>GGHMKNILVTGGLGFIGSNFVNHISSKYDNVNIYVYDIGDYCASVENVEWNNRTKLIKGDIRNFDLIMHTLT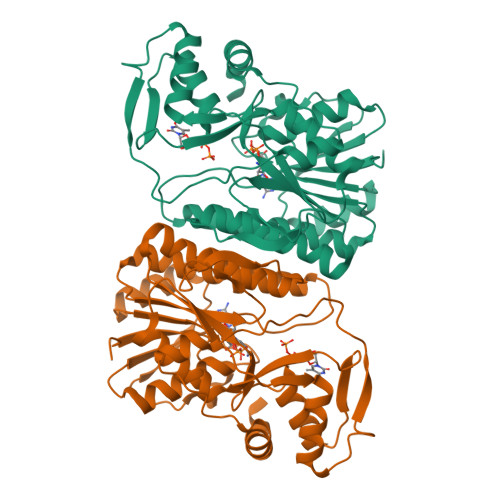EHEIDTIVHFAAHSHVDNSFKNSLAFTETNVFGTHVLLECSRMYGKLKLFFHMSTDEVYGEIDTTDTSREVSLLCPTNPYAATKAGAEHIVKSYFLSYKLPIIIARCNNVYGRNQYPEKLIPKFICSLLDGKKLHIQGTGNSRRNFIHAIDVADAVDLVINNGVIGETYNIGVTNEHSVLDVAQILCDIAGVNLENQLEYVPDRLFNDFRYNITNDKIKSLGWEQSRKDFKKELVELFDWYKVNRHRYNIPGSQ[4x]>[3x]MLEANVYDNFNPNYYNISDFSMPNGKKEKRGLPIPKARCQVINYELWETGYLYTSSATLTVSVEVGDIVQILFPEVVPIEEALGKKKKLNLDMVYLVTDVDESNKATLKNYFWAMIESLDVPNAITKTTNFAIIDYLIDPNKNNLMSYGYFFNSSIFAGKATINRKAETSSAHDVAKRIFSKVQFQPTTTIQHAPSETDPRNLLFINFASRNWNRKRITTRVDIKQSVTMDTETIVDRSAYNFAVVFVKNKATDD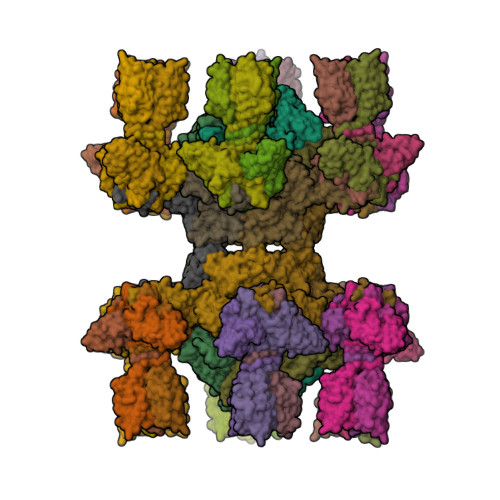YTDPPKMYIAKNNGDVIDYSTYHGDGTDLPDVRTAKTLFYDRDDHGNPPELSTIKVEISPSTIVTRLIFNQNELLPLYVNDLVDIWYEGKLYSGYIADRVKTEFNDRLIFVESGDKPNVI;>[18x]TIKNFTFFSPNSTEFPVGSNNDGKLYMMLTGMDYRTIRRKDWSSPLNTALNVQYTNTSIIAGGRYFELLNETVALKGDSVNYIHANIDLTQTANPVSLSAETANNSNGVDINNGSGVLKVCFDIVTTSGTGVTSTKPIVQTSTLDSISVNDMTVSGSIDVPVQTLTVEAGNGLQLQLTKKNNDLVIVRFFGSVSNIQKGWNMSGTWVDRPFRPAAVQSLVGHFAGRDTSFHIDINPNGSITWWGANIDKTPIATRGNGSYFIK;>GVRQYKIHTNLDGTDDKVWDVTNGKVRFYQPSNLGLQSTNNIWQSNGIGVMGTRSITQPQIEFKLETFGESLEENYQLMKDFVNDILSKKFVTLEYQTEIFQVYADLALADVTKTEGYGKNGTFSEKITFDIITKWYTYENLTFDKIQNGKVIAGMSKIYGGTAPGNYKYIKGTSYTYYGESDIDRLSRWDIKEEIFSFMGILYPKLPKTPAGVRFLDDIGNEYTAIVFKTEQVQDYILINTDVNDETYQGWKGTTALNLFPVMDFERYRTRIIEKGQMELINLSKAEFKIKRKADFV[6x]>[4x]GAHMVSVIKPEMKMRYYMDGSVNGHEFTIEG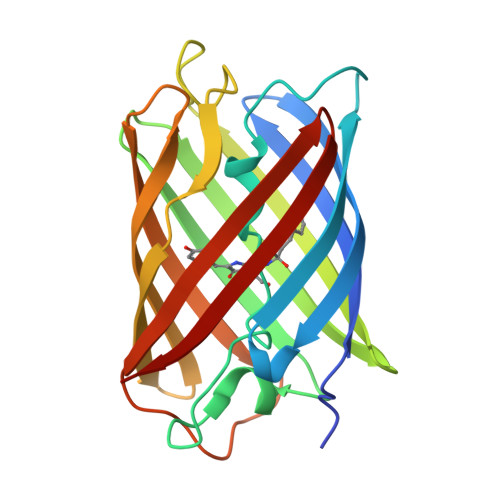EGTGRPYEGHQEMTLRVTMAKGGPMPFAFDLVSHVFCYGHRPFTKYPEEIPDYFKQAFPEGLSWERSLEFEDGGSASVSAHISLRGNTFYHKSKFTGVNFPADGPIMQNQSVDWEPSTEKITASDGVLKGDVTMYLKLEGGGNHKCQFKTTYKAAKKILKMPGSHYISHRLVRKTEGNITELVEDAVAHS>GHMEQTHRAIFRFVPRHEDELELEVDDPLLVELQAEDYWYEAYNMRTGARGVFPLYYAIEVTK[4x]

Aromatic residues cluster in the core of folded proteins, where they stabilize the structure through multiple interactions. NMR studies in the 1970s demonstrated that aromatic side chains can undergo ring flips—that is, 180° rotations of the χ2 dihedral angle (Cβ–Cγ axis)—even when engaged in stabilizing interactions in the hydrophobic core. Here we capture ring flipping events of a buried tyrosine residue in the SH3 domain of the JNK-interacting protein 1 (JIP1). Our data therefore suggest that the conformation of the aromatic ring at position 526 is determined by steric interactions dictated by the size of the surrounding amino acids.

Accordingly, we designed four different mutants of JIP1-SH3 (H493A, V517A, V517L and A541L) and obtained their high-resolution structures by X-ray crystallography. Of note, three mutants (H493A, V517A and A541L) induce a staggered conformation of Y526, with χ2 dihedral angles ranging from −41° to −75°, whereas V517L shows an eclipsed conformation of Y526 and an almost identical structure to the wild-type protein. The A541L mutation also triggers a staggered conformation of Y526 and a rearrangement of the 517–522 region; however, the stabilization mechanism of the aromatic ring is different. A looping out of the β-strand between residues 517 and 522 is observed, which allows the side chain of A521 to reorient and to stabilize the staggered conformation of the ring through CH–π interactions together with L541 and V517. At the same time, the side chains of L519, Q520 and E522 and D523 undergo large-scale movements to accommodate the flipped ring within the pocket. The initial generation of void volume around the ring is almost identical along the structural trajectory between the major state (wild type) and the A541L crystal structure. Thus, all mutants—including A541L, which stabilizes Y526 in a staggered conformation by a different mechanism—share the same initial structural trajectory and report on identical breathing motions.> GKNTPKSAIIYTTMGDIHISLFYKECKKTVQNFSVHSINGYYNNCIFHRVIKHFMVQTGDPSGDGTGGESIWGNEFEDEFFDHLNHSKPFMVSMANCGPNTNGSQFFITTVPCPWLDFKH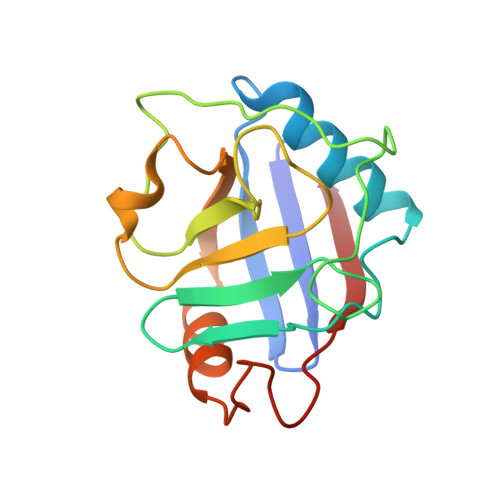TVFGKVTQGSKIVLDIEKVRTDKRDKPLEDIKILNIKINN> MERNRLARQIIDTCLEMTRLGLNQGTAGNVSVRYQGGMLITPTGIPYEKLTEDKIVFIDADGQHEQGKLPSSEWRFHQAAYQTRPDAQAVVHNHA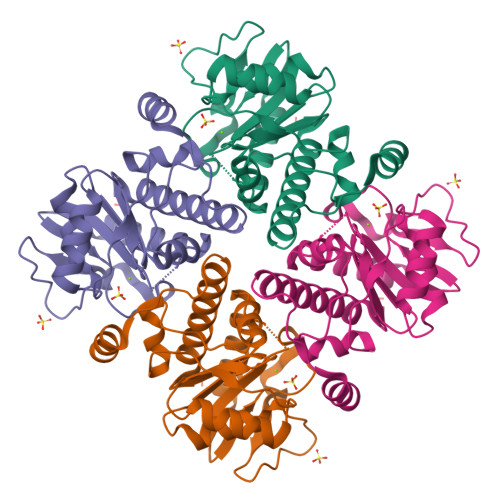VHCTAVSILNRPIPAIHYMIAAAGGNSIPCAPYATFGTRELSEHVAVALKHRKATLLQHHGLIACEASLEKALWLAHEVEVLAQLYLSTLAITDPVPVLDDEAIAIVLEKFKTYGLRIEE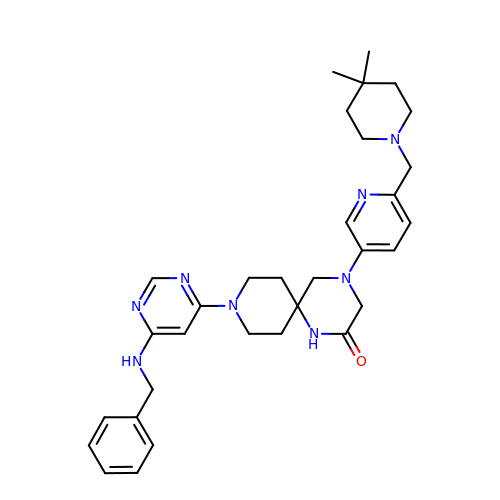4-[6-[(4,4-dimethylpiperidin-1-yl)methyl]pyridin-3-yl]-9-[6-[(phenylmethyl)amino]pyrimidin-4-yl]-1,4,9-triazaspiro[5.5]undecan-2-one | C32 H42 N8 O | LSPKIAXMFJWAHQ-UHFFFAOYSA-N>GYLLGSA[2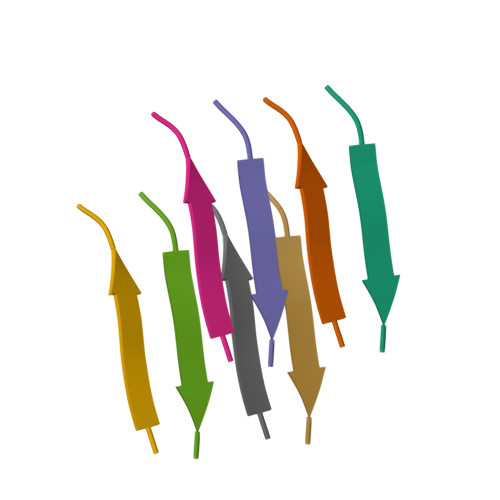x]> EKEERTWQDEAIYFIMVDRFNNMDPTNDQNVNVNDPKGYFGGDLKGVTAKLDYIKEMGFTAIWLTPIFKNMP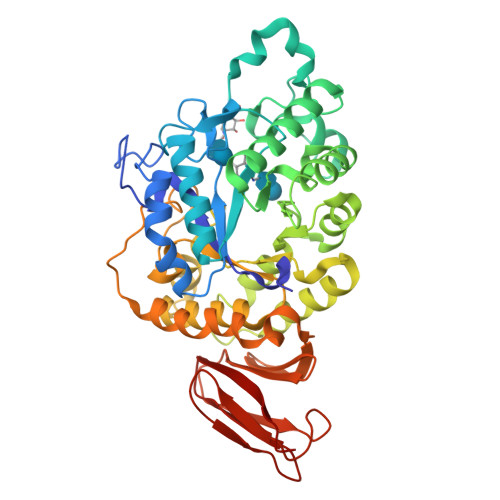GGYHGYWIEDFYQVDPHFGTLGDLKTLVKEAHKRDMKVILDFVANHVGYNHPWLHDPTKKDWFHPKKEIFDWNDQTQLENGWVYGLPDLAQENPEVKTYLIDAAKWWIKETDIDGYRLDTVRHVPKSFWQEFAKEVKSVKKDFFLLGEVWSDDPRYIADYGKYGIDGFVDYPLYGAVKQSLARRDASLRPLYDVWEYNKTFYDRPYLLGSFLDNHDTVRFTKLAIDNRNNPISRIKLAMTYLFTAPGIPIMYYGTEIAMNGGQDPDNRRLMDFRADPEIIDYLKKIGPLRQELPSLRRGDFTLLYEKDGMAVLKRQYQDETTVIAINNTSETQHVHLTNDQLPKNKELRGFLLDDLVRGDEDGYDLVLDRETAEVYKLREKT(3S)-1-({[(3S)-piperidin-3-yl]oxy}acetyl)-N-({4-[4-(trifluoromethyl)phenyl]-1,3-thiazol-2-yl}methyl)piperidine-3-carboxamide 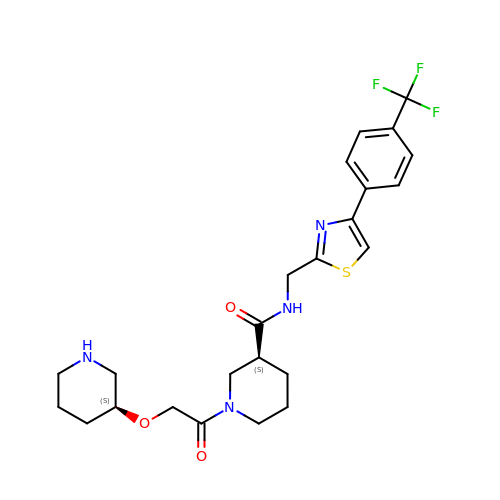| C24 H29 F3 N4 O3 S | OVPLOMYZPJLWSF-HKUYNNGSSA-N> MKHHHHHHSAGLEVLFQGPGTGSEFELMMFGKKKNNGGSSTARYSAGNKYNTLSNNYALSAQQLLNASKIDDIDSMMGFERYVPPQYNGRFDAKDIDQIPGRVGWLTNMHATLVSQETLSSGSNGGGNSNDGERVTTNQGISGVDFYFLDEEGGSFKSTVVYDPYFFIACNDESRVNDVEELVKKYLESCLKSLQIIRKEDLTMDNHLLGLQKTLIKLSFVNSNQLFEARKLLRPILQDNANNNVQRNIYNVAANGSEKVDAKHLIEDIREYDVPYHVRVSIDKDIRVGKWYKVTQQGFIEDTRKIAFADPVVMAFAIATTKPPLKFPDSAVDQIMMISYMIDGEGFLITNREIISEDIEDFEYTPKPEYPGFFTIFNENDEVALLQRFFEHIRDVRPTVISTFNGDFFDWPFIHNRSKIHGLDMFDEIGFAPDAEGEYKSSYCSHMDCFRWVKRDSYLPQGSQGLKAVTQSKLGYNPIELDPELMTPYAFEKPQHLSEYSVSDAVATYYLYMKYVHPFIFSLCTIIPLNPDETLR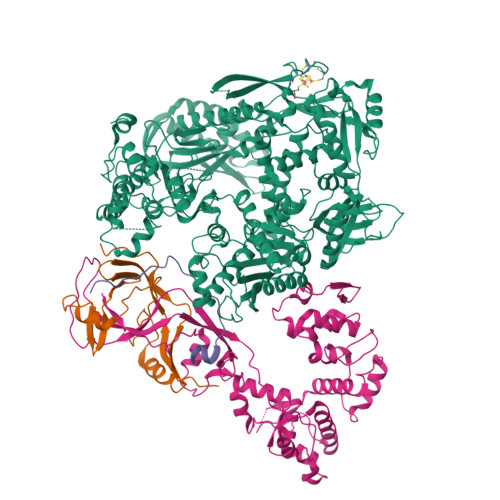KGTGTLCEMLLMVQAYQHNILLPNKHTDPIERFYDGHLLESETYVGGHVESLEAGVFRSDLKNEFKIDPSAIDELLQELPEALKFSVEVENKSSVDKVTNFEEIKNQITQKLLELKENNIRNELPLIYHVDVASMYPNIMTTNRLQPDSIKAERDCASCDFNRPGKTCARKLKWAWRGEFFPSKMDEYNMIKRALQNETFPNKNKFSKKKVLTFDELSYADQVIHIKKRLTEYSRKVYHRVKVSEIVEREAIVCQRENPFYVDTVKSFRDRRYEFKGLAKTWKGNLSKIDPSDKHARDEAKKMIVLYDSLQLAHKVILNSFYGYVMRKGSRWYSMEMAGITCLTGATIIQMARALVERVGRPLELDTDGIWCILPKSFPETYFFTLENGKKLYLSYPCSMLNYRVHQKFTNHQYQELKDPLNYIYETHSENTIFFEVDGPYKAMILPSSKEEGKGIKKRYAVFNEDGSLAELKGFELKRRGELQLIKNFQSDIFKVFLEGDTLEGCYSAVASVCNRWLDVLDSHGLMLEDEDLVSLICENRSMSKTLKEYEGQKSTSITTARRLGDFLGEDMVKDKGLQCKYIISSKPFNAPVTERAIPVAIFSADIPIKRSFLRRWTLDPSLEDLDIRTIIDWGYYRERLGSAIQKIITIPAALQGVSNPVPRVEHPDWLKRKIATKEDKFK;> MSINLHSAPEYDPSYKLIQLTPELLDIIQDPVQNHQLRFKSLDKDKSEVVLCSHDKTWVLKQRKHSNTVLLMREFVPEQPITFDETLLFGLSKPYMDVVGFAKTESEFETRETHGELNLNSVPIYNGELDFSDKIMKRSSTKVIGTLEELLENSPCSALEGISKWHKIGGSVKDGVLCILSQDFLFKALHVLLMSAMAESLDLQHLNVEDTHHAVGKDIEDEFNPYTREIIETVLNKFAVQEQEAENNTWRLRIPFIAQWYGIQALRKYVSGISMPIDEFLIKWKSLFPPFFPCDIDIDMLRGYHFKPTDKTVQYIAKSTLPMDPKERFKVLFRLQSQWDLEDIKPLIEELNSRGMKIDSFIMKYARRKRLGKKTVVTSR;> MPSVDIDASQWQKLTQSREKQTTVITPLGMMMLEIQGELELPKDFASLARRDSPNEGRFSEQDGETLIRFGSLQIDGERATLFVGKKQRLLGKVTKLDVPMGIMHFNSKDNKVELVDVMKYKVIFKDRPLPIM;> GAMGNQTVKIWVKYNEGFSNAVRKNVTWNNLWE> MKKNGKSQNQPLDFTQYAKNMRKDLSNQDICLEDGALNHSYFLTKKGQYWTPLNQKALQRGIELFGVGNWKEINYDEFSGKANIVELELRTCMILGINDI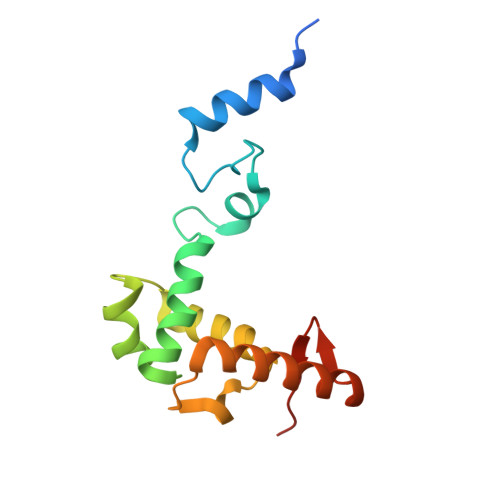TEYYGKKISEEEQEEIKKSNIAKGKKENKLKDNIYQKLQQMQ>KGQEV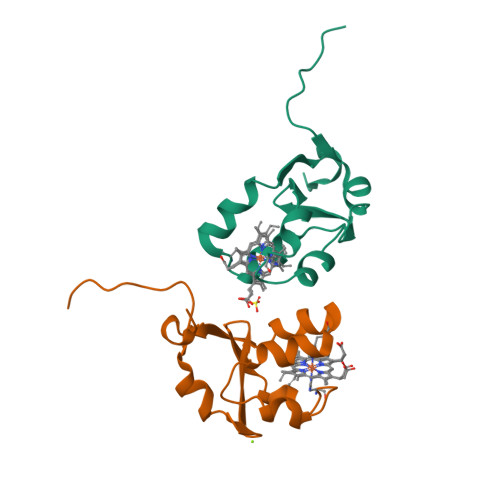ETSVTYYRLEEVAKRNSLKELWLVIHGRVYDVTRFLNEHPGGEEVLLEQAGVDASESFEDVGHSSDAREMLKQYYIGDIHPSDLKPE[2x]3-[(4-hydroxy-2-methylpyrimidin-5-yl)methyl]-5-(2-{[(R)-hydroxy(phosphonooxy)phosphoryl]oxy}ethyl)-4-methyl-1,3-thiazol-3-ium | C12 H18 N3 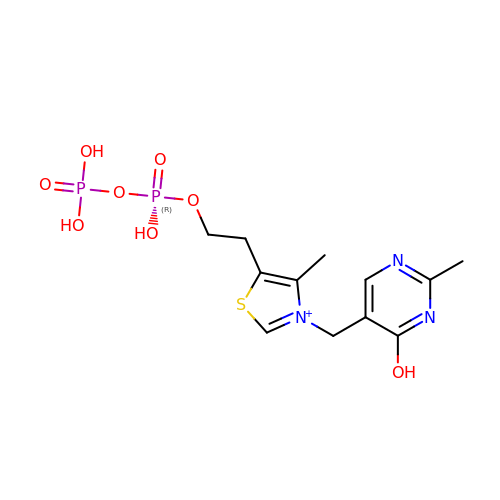O8 P2 S | FBFAORFKQFQJGN-UHFFFAOYSA-O>[2x]MGAAILPDLGTEILIPVCAVIGIAFALFQWLLVSKVKLSAVRDASPNAAAKNGYNDYLIEEEEGINDHNVVVKCAEIQNAISEGATSFLFTEYKYVGIFMVAFAILIFLFLGSVEGFSTSPQACSYDKTKTCKPALATAIFSTVSFLLGGVTSLVSGFLGMKIATYANARTTLEARKGVGKAFITAFRSGAVMGFLLAANGLLVLYIAINLFKIYYGDDWGGLFEAIDGYGLGGSSMALFGRVGGGIYTKAADVGADLVGKVERNIPEDDP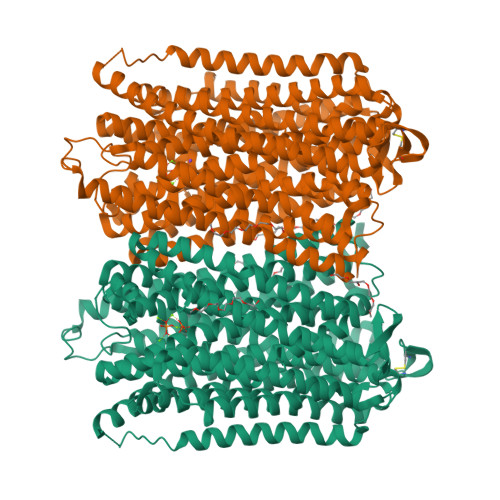RNPAVIADNVGDNVGDIAGMGSDLFGSYAESSCAALVVASISSFGLNHELTAMLYPLIVSSVGILVCLLTTLFATDFFEIKAVKEIEPALKKQLVISTVLMTIGVAVVSFVALPTSFTIFNFGVQKDVKSWQLFLCVAVGLWAGLIIGFVTEYYTSNAYSPVQDVADSCRTGAATNVIFGLALGYKSVIIPIFAIAISIFVSFTFAAMYGIAVAALGMLSTIATGLAIDAYGPISDNAGGIAEMAGMSHRIRERTDALDAAGNTTAAIGKGFAIGSAALVSLALFGAFVSRASITTVDVLTPKVFIGLIVGAMLPYWFSAMTMKSVGSAALKMVEEVRRQFNTIPGLMEGTAKPDYATCVKISTDASIKEMIPPGALVMLTPLVVGILFGVETLSGVLAGSLVSGVQIAISASNTGGAWDNAKKYIEAGASEHARSLGPKGSDCHKAAVIGDTIGDPLKDTSGPSLNILIKLMAVESLVFAPFFATHGGLLFKIF> GSRRASVGAHMIFAVRTMV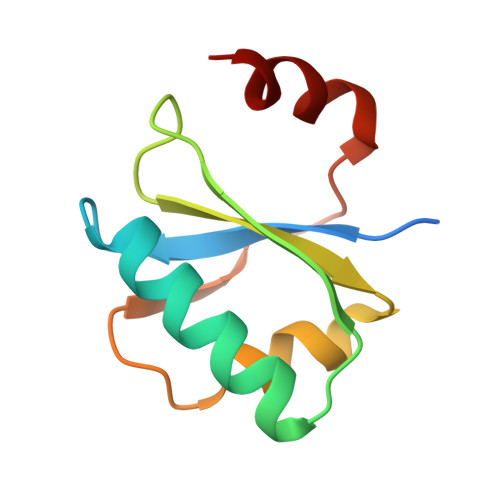GQEKNIAGLMASRAEKEQLDVYSILASESLKGYVLVEAETKGDVEELIKGMPRVRGIVPGTIAIEEIEPLLTP{(3R,4R)-4-methyl-3-[methyl(7H-pyrrolo[2,3-d]pyrimidin-4-yl)amino]piperidin-1-yl}[(3R)-3-(phenylsulfonyl)pyrrolidin-1-yl]methanone 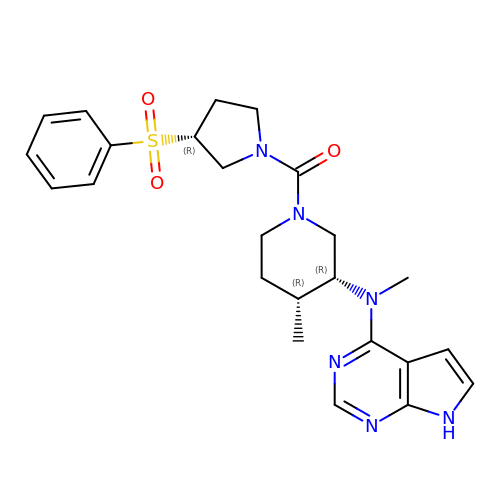| C24 H30 N6 O3 S | XEFTYQOQZCRKHD-QFUCXCTJSA-N> MAYPYSDMPFGVELDTSTLGSFGL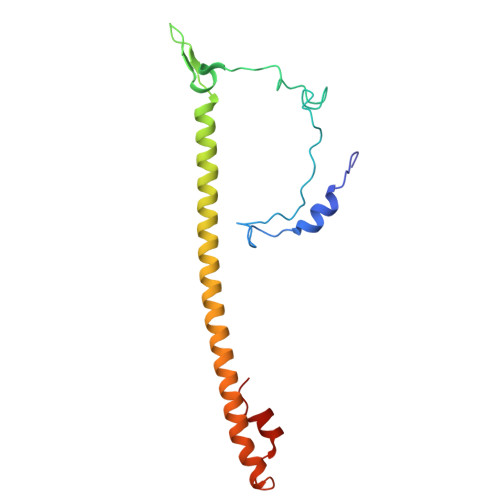GGPQTQLQMQMPAVDVNAAASGSGGFMAGFSNIFSRDSMFGGVAPSGAQTGGWVLPALGIGQAVFGAIGANRQQRAARDQLAESRRQFDMNYGAQRQSINTNLEDRQRARVASNPTAYESVDSYMERNRIR> GSHMIKIGAHMPISKGFDRVPQDTVNIGGNSFQIFPHNARSWSAKLPSDEAATKFKREMKKHGIDWENAFCH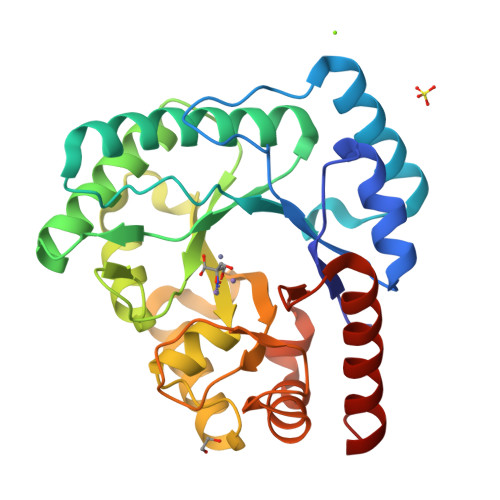SGYLINLASPKDDIWQKSVELLKKEVEICRKLGIRYLNIHPGSHLGTGEEEGIDRIVRGLNEVLNNTEGVVILLENVSQKGGNIGYKLEQLKKIRDLVDQRDRVAITYDTCHGFDSGYDITKKEGVEALLNEIESLFGLERLKMIHLNDSKYPLGAAKDRHERIGSGFIGEEGFAVFFSFKEIQEVPWILETPGGNEEHAEDIKKVFEIIEKFGIE> MTDIYIPPEGLYFRLLGFASRQVIFARNSPSPDVGLSPVNDQATDQYFSLI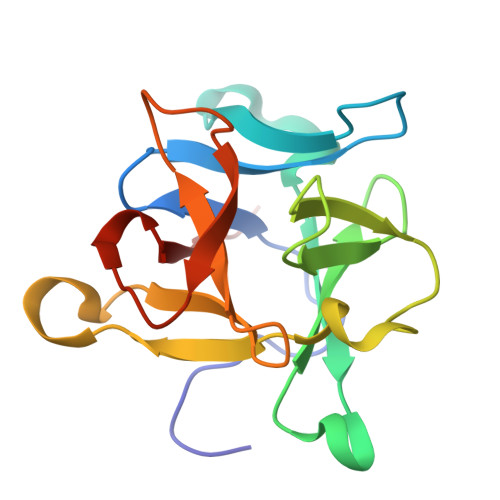YGTGEHAGLYAIKSKATGKVLFSRRPAEPYVGQIDGDGRYPDNWFKIEPGKTYLSKYFRLVQPSTGTALVSRTHLQPYFWNHPQTEVFDDQYFTFLFED>[2x]MIDCAIIGGGPAGLSAGLYATRGGVKNAVLFEKGMPGGQITGSSEIENYPGVKEVVSGLDFMQPWQEQCFRFGLKHEMTAVQRVSKKDSHFVIL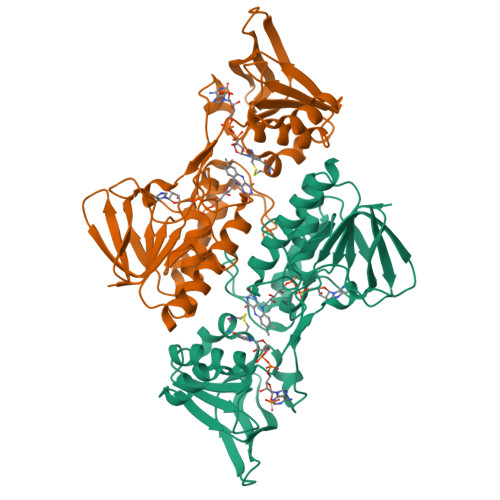AEDGKTFEAKSVIIATGGSPKRTGIKGESEYWGKGVSTCATCDGFFYKNKEVAVLGGGDTAVEEAIYLANICKKVYLIHRRDGFRCAPITLEHAKNNDKIEFLTPYVVEEIKGDASGVSSLSIKNTATNEKRELVVPGFFIFVGYDVNNAVLKQEDNSMLCKCDEYGSIVVDFSMKTNVQGLFAAGDIRIFAPKQVVCAASDGATAALSVISYLEHH>[2x]GPHMKTHIDDYSTWDIVKATQYGIYERCRELVEAGYDVRQPDKENVTLLHWAAINNRIDLVKYYISKGA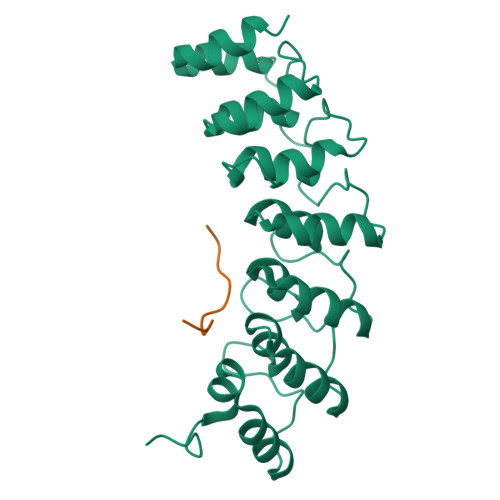IVDQLGGDLNSTPLHWATRQGHLSMVVQLMKYGADPSLIDGEGCSCIHLAAQFGHTSIVAYLIAKGQDVDMMDQNGMTPLMWAAYRTHSVDPTRLLLTFNVSVNLGDKYHKNTALHWAVLAGNTTVISLLLEAGANVDAQNIKGESALDLAKQRKNVWMINHLQEARQAK;>[2x]GVVASQPARV>MHHHHHHEENVKRRT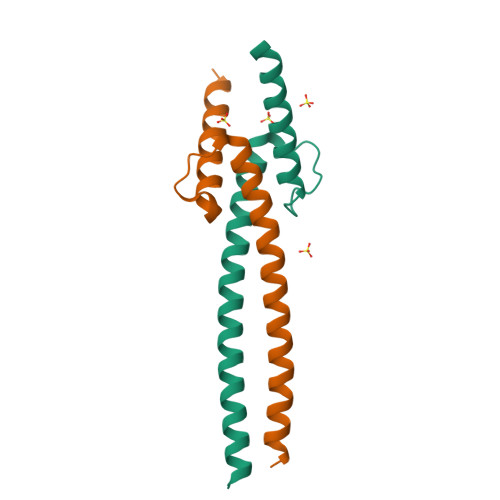HNVLERQRRNELKRSFFALRDQIPELENNEKAPKVVILKKATAYILSVQAEEQKLISEEDLLRKRREQLKHKLEQLRNS[2x];>[2x]MADKRAHHNALERKRRDHIKDSFHSLRDSVPSLQGEKASRAQILDKATEYIQYMRRKNHTHQQDIDDLKRQNALLEQQVRALE> 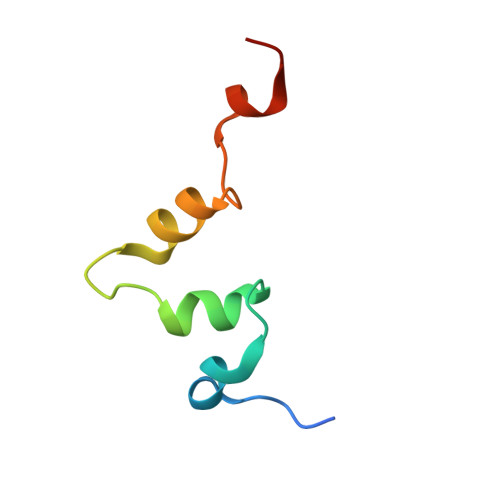GSAIKVVKPSDWDSLPDTDLRYIYSQRQPEKTMHERLKGKGVIVDMASLFKQAG> GSHMSGIALSRLAQERKAWRKDHPFGFVAVPTKNPDGTMNLMNWECAIPGKKGTPWEGGLFKLRMLFKDDYPSSPPKCKFEPPLFHPQVYPSGTVCLSILEEDKDWRPAITIK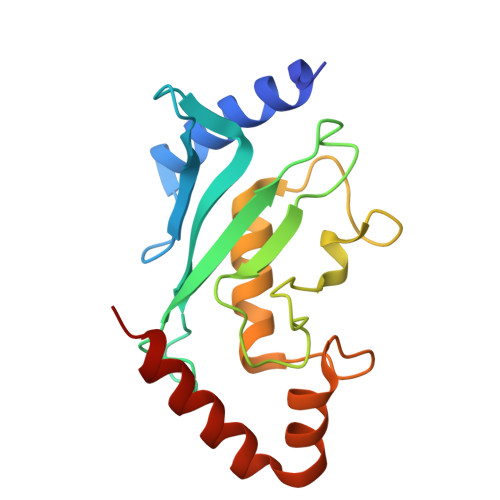QILLGIQELLNEPNIQDPAQAEAYTIYCQNRVEYEKRVRAQAKKFAPS> FSAQT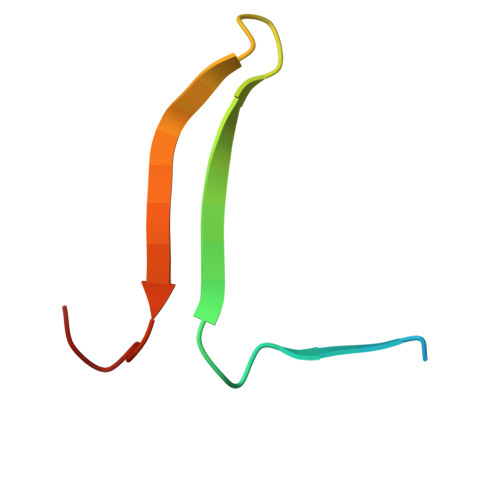NRHILRFNRPFLVVIFSTSTQSVLFLGKVVDPTKP>SLEKQIESYYQEIAQLIIDMIPEEWAEVRFYAQEDHDGWKIFFFHYLSASSDEWTKDIDIRDVIKVPQDEFMEKYNELSFCISDFRKDYAEAFGEPWMSFQMTFYASGKFNIDFYYDKNPFDTFLTRLAWQYEHFGTIPEDSFYKETLNEYLEEKAQ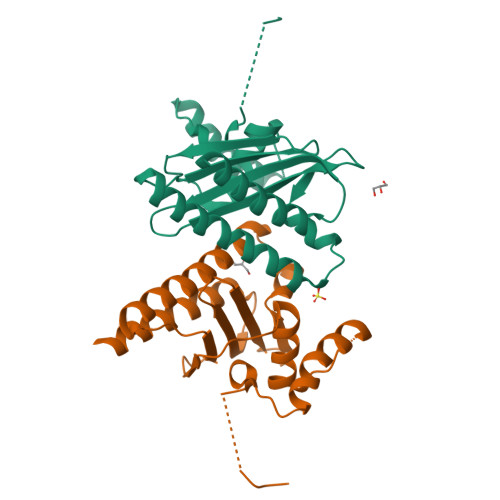GKRYPFLEPLKEEEGHHHHHH[2x]(2E)-N-benzyl-2-cyano-3-(pyridin-4-yl)prop-2-enamide | C16 H13 N3 O | 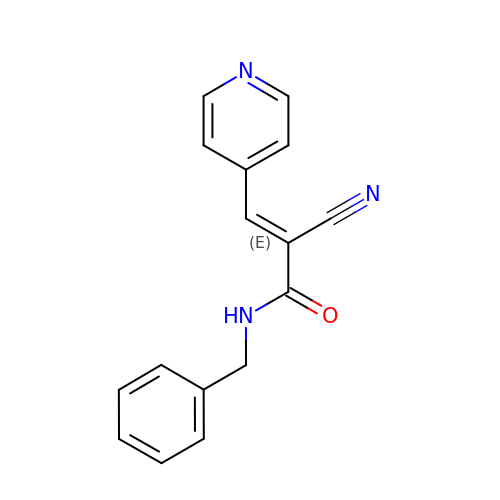JGNYTGFSGUFNSH-XNTDXEJSSA-N> RVSIGGTVYT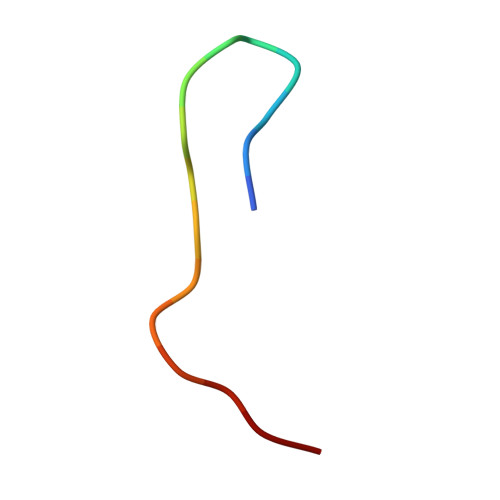AKKYDD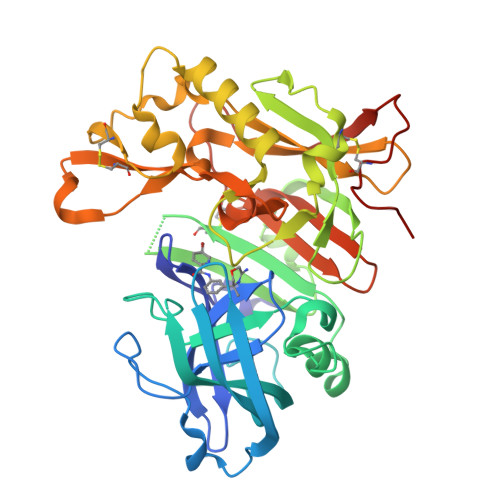> GPFVEMVDNLRGKSGQGYYVEMTVGSPPQTLNILVDTGSSNFAVGAAPHPFLHRYYQRQLSSTYRDLRKGVYVPYTQGKWEGELGTDLVSIPHGPNVTVRANIAAITESDKFFINGSNWEGILGLAYAEIARPDDSLEPFFDSLVKQTHVPNLFSLQLCGAGFPLNQSEVLASVGGSMIIGGIDHSLYTGSLWYTPIRREWYYEVIIVRVEINGQDLKMDCKEYNYDKSIVDSGTTNLRLPKKVFEAAVKSIKAASSTEKFPDGFWLGEQLVCWQAGTTPWNIFPVISLYLMGEVTNQSFRITILPQQYLRPVEDVATSQDDCYKFAISQSSTGTVMGAVIMEGFYVVFDRARKRIGFAVSACHVHDEFRTAAVEGPFVTLDMEDCGYNIPQTDES> AAAAFAFF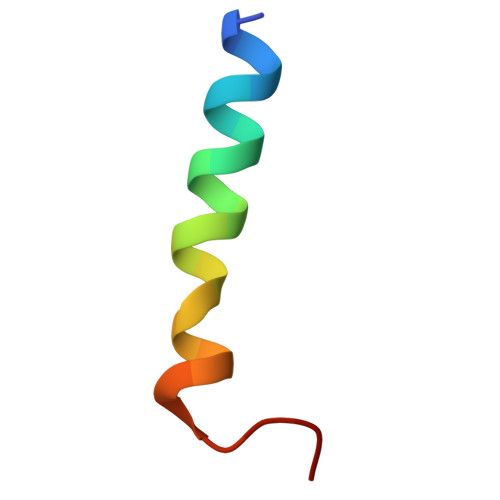AGFAFAAFAAAAAAAA> DAMIVIDGHGIIQLFSTAAERLFGWSELEAIGQNVNILMPEPDRSRHDSYISRYRTTSDPHIIGIGRIVTGKRRDGTTFPMHLSIGEMQSGGEPYFTGFVRDLTEHQQ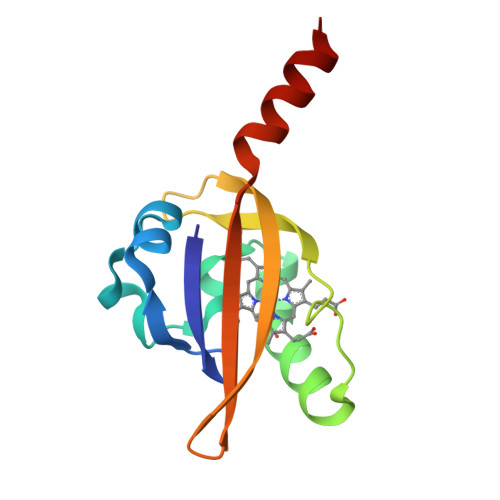TQARLQEL1~{H}-imidazole-2,4-diol | C3 H4 N2 O2 | 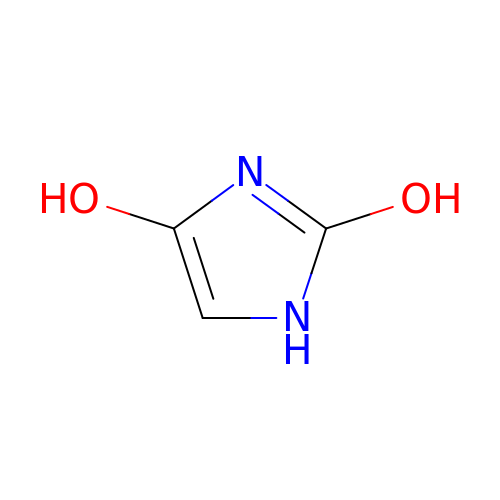SHFCYMWGNNAKEL-UHFFFAOYSA-N> GFKDYGHDYHPAPKTENIKGLGDLKPGIPKTPKQNGGGKRKRWTGDKGRKIYEWDSQHGELEGYRAS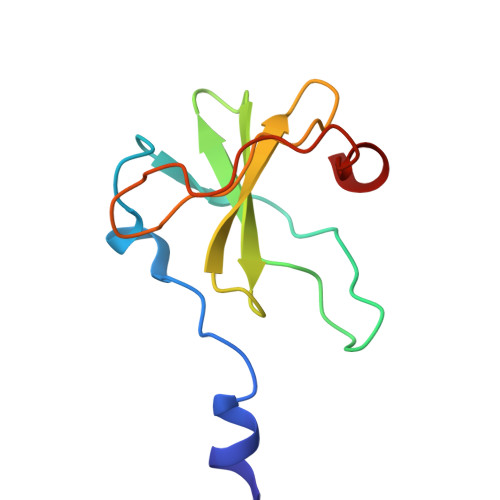DGQHLGSFDPKTGNQLKGPDPKRNIKKYL>[10x]MSLINTKIKPFKNQAFKNGEFIEITEKDTEGRWSVFFFYPADFTFVCPTELGDVADHYEELQKLGVDVYAVS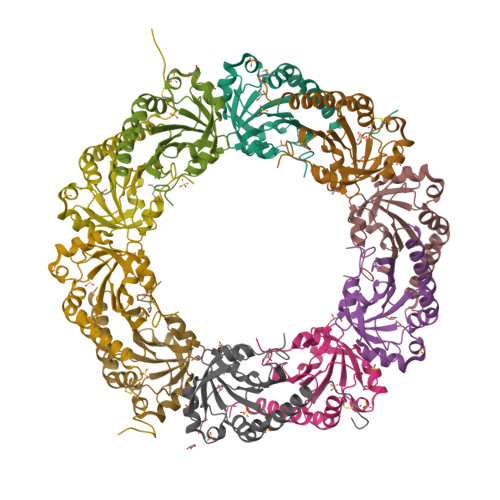TDTHFTHKAWHSSSETIAKIKYAMIGDPTGALTRNFDNMREDEGLADRATFVVDPQGIIQAIEVTAEGIGRDASDLLRKIKAAQYVASHPGEVCPAKWKEGEATLAPSLDLVGKYFSKHN5-FLUORO-4-[(1S)-1-(5-FLUOROPYRIMIDIN-2-YL)ETHOXY]-N-(5-METHYL-1H-PYRAZOL-3-YL)-6-MORPHOLINO-PYRIMIDIN-2-AMINE | 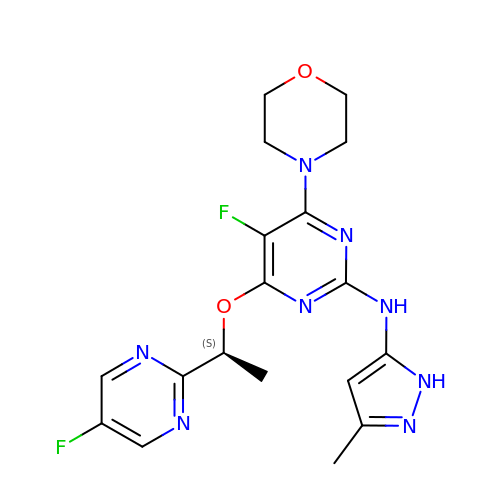C18 H20 F2 N8 O2 | NFYAORHLODKCQX-NSHDSACASA-N>[4x]MDKLPPSMRKRLYSLPQQVGAKAWIMDEEEDAEEEGAGGRQDPRRRSIRLRPLPSPSPSPSAAAAAAGGAESRGAALGGAADGEGPARGAAKSSTNGDCRRFRGSLASLGSRGGGGGGGSTGGGSHGHLHDSAEERRLIAEGDASPGEDRTPPGLAAEPERPGAPAPPAASPPQVPSSCGEQRPADAAVKVEGGAAAGDQILPEAEARLGQAGFMQRQFGAMLQPGVNKFSLRMFGSQKAVEREQERVKSAGFWIIHPYSDFRFYWDLTMLLLMVGNLIIIPVGITFFKDENTTPWIVFNVVSDTFFLIDLVLNFRTGIVVEDNTDIILDPRRIKMKYLKSWFVVDFVSSIPVDYIFLIVETRIDSEVYKTARALRIVRFTKILSLLRLLRLSRLIRYIHQWEEIFHMTYDLASAVVRIVNLIGMMLLLCHWDGCLQFLVPMLQDFPDDCWVSLNNMVNNSWGKQYSYALFKAMSHMLCIGYGRQAPMGMSDVWLTMLSMIVGA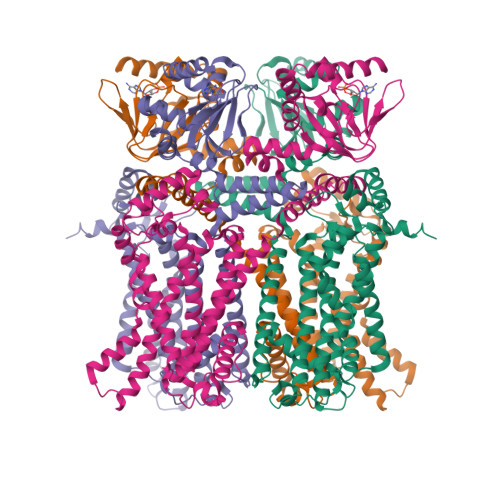TCYAMFIGHATALIQSLDSSRRQYQEKYKQVEQYMSFHKLPPDTRQRIHDYYEHRYQGKMFDEESILGELSEPLREEIINFNCRKLVASMPLFANADPNFVTSMLTKLRFEVFQPGDYIIREGTIGKKMYFIQHGVVSVLTKGNKETKLADGSYFGEICLLTRGRRTASVRADTYCRLYSLSVDNFNEVLEEYPMMRRAFETVALDRLDRIGKKNSIHKVQHDLSSGVSNYQENAIVQRIVQHDREMAHCARRAQATTPVAPAIWTPLIQAPLQAAAQDLKLISASQPALPQDGAQTLRRASPHSSSGESVAALPPAGGPFPRAPGRPPGAGPGQHVTLTLPRKASSGSLPPPLSLFGPRAAPRLTAAPQREPGAKSEPVRSKLPSNL> APVRSLNCTLRDSQQKSLVMSGPYELKALHLQGQDMEQQVVFSMSFVQGEESNDKIPVALGLKEKNLYLSSVLKDDKPTLQLESVDPKNYPKK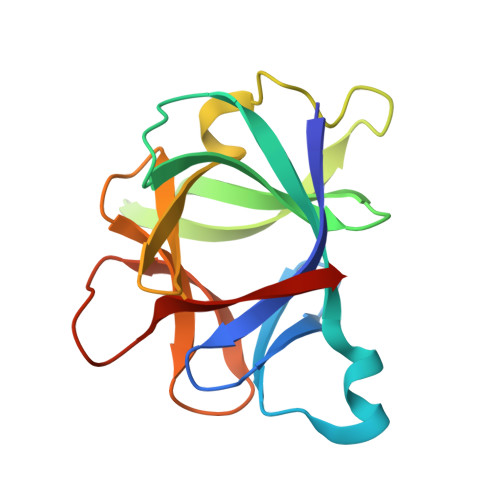KMEKRFVFNKIEINNKLEFESAQFPNWYISTSQAENMPVFLGGTKGGQDITDFTMQFVSS>MSSGKKP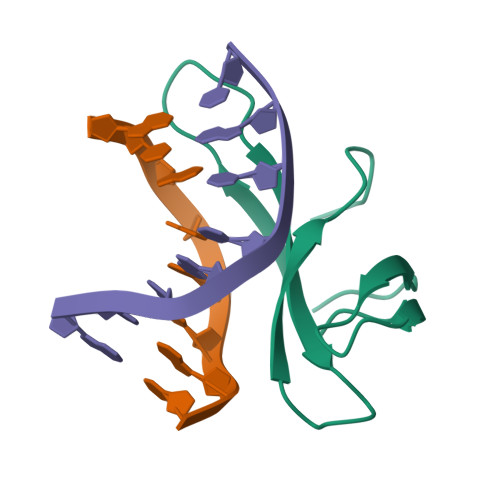VKVKTPAGKEAELVPEKVWAAAPKGRKGVKIGLFKDPETGKYFRHKLPDDYPI[2x]Transcription factors (TFs) recognize specific bases within their DNA-binding motifs, with each base contributing nearly independently to total binding energy. However, the energetic contributions of particular dinucleotides can deviate strongly from the additive approximation, indicating that some TFs can specifically recognize DNA dinucleotides. Here we solved high-resolution (<1 Å) structures of MYF5 and BARHL2 bound to DNAs containing sets of dinucleotides that have different affinities to the proteins. The dinucleotides were recognized either enthalpically, by an extensive water network that connects the adjacent bases to the TF, or entropically, by a hydrophobic patch that maintained interfacial water mobility.

To understand why both possible single base substitutions of AC that make it more similar to TT (AT and TC) lead to a decrease in affinity, we first investigated why DNAAT has a lower affinity to BARHL2 than both optimal sequences. The DNA recognition pattern in the BARHL2–DNAAT complex is more similar to DNAAC than DNATT. Compared to DNAAC, the hydrophobic contact between Thr285 and T18 opposite to A7 of AC is retained, but the extensive water network connecting both Thr285 and Thr278 with the AC region is almost completely lost. There is only one water molecule connecting the side-chain oxygen of Thr285 with the side-chain oxygen of Asn282 and one water molecule connecting Asn282 with N6 of A7 of AC. In addition, the side chain of Arg289 has only one conformation, rotated away from the protein–DNA interface.

>KPRKARTAFSDHQLNQLERSFERQKYLSVQDRMDLAAALNLTDTQVKTWYQNRRTKWKRQTA[6x]> GPHMSTSSANEDMPVEKILEAELAVEPKTETYVEANMGLNPSSPNDPVTNICQAADKQLFTLVEWAKRIPHFSELPLDDQVILLRAGWNELLIASFSHESIAVKDGILLATGLHVHRNSAHSAGVGAIFDRVLTELVSKMRD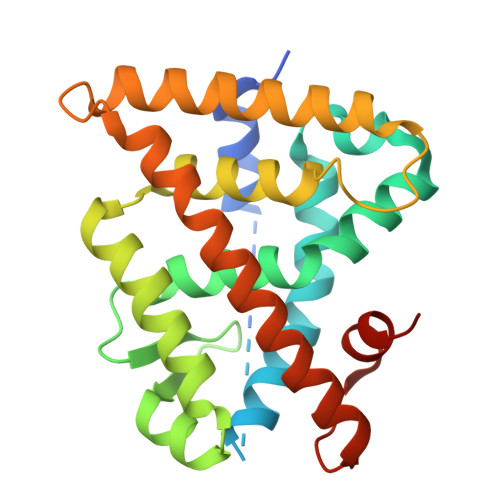MQMDKTELGCLRAIVLFNPDSKGLSNPAEVEALREKVYASLEAYCKHKYPEQPGRFAKLLLRLPALRSIGLKQLEHLFFFKLIGDTPIDTFLMEMLEAPHQAT> KQGPTSVAYVEVNNNSMLNVGKYTLADGGGNAFDVAVIFAANINYDTGTKTAYLHFNENVQRVLDNAVTQIRPLQQQGIKVLLSVLGNHQGAGFANFPSQQAASAFAKQLSDAVAKYGLDGVDFDDAYAEYGNNGTAQPNDSSFVHLVTALRANMPDKIISLYNIGPAASRLSYGGVDVSDKFDYAWNPYYGTWQVPGIALP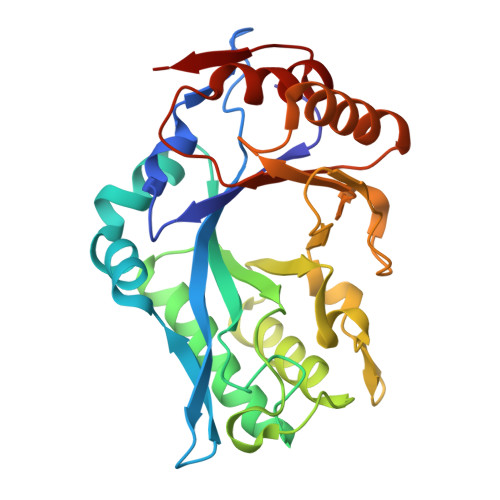KAQLSPAAVEIGRTSRSTVADLARRTVDEGYGVYLTYNLDGGDRTADVSAFTRELYGSEAVRT>MISKRIARLSDKVRNTQPTIDLDRARLITEFYSRPSMDNYILRRAKAFDYYLENREIFIDEDSQIAGHQGGCWEAVVMHPDVTKWLYDDFDTLDKRPSDNLAFRSAAAKEELRQIVETWKGQTFGDFAATLVDEDMKPMLDVGIFTHGISNQSTMNHSPDYDNLIKRGYRYYIDECKEKLAEHQVNDVYDMEQQIAWKAMIIAMEAVIKFAHRYADLANKQAAECIDPKRKEELLIMAENCRTVPENPPKTFLQATQLVWFNHLAISLEAAGGDHNLGRYDQYMLPFFEKETAEGKPEEYFADIIHEFKLKVAEMWNIRCYNESVADPGNPLWMHIMLAGQLENGKDACNELTNVFLRCMRDLQTDEPCITFRFHPNINEETFRLAIEVARDSGGHPAFYNDTAAITYLLSLGFTLKEARNWGICGCIEPQVLGKTDFQSNPGYFNPLKVFDVMLHNGYDPVIGKKIGIESGEVSSFTSIDDVMRAYEKQLDFFMEKFVTLANRTLAGHAFTLPTIMGSCFSVGCVEKGKLLQQKGSDHHYSAVGVAGIANMIDSFAAMEECVFNKNYLTMEELVRLLDTNFEGKENMRQLLLNKAPKFGNDIEQVDKYSYWLIDALDTSMKRFHDAQGGPYTVLVATQAYNVEMGKNVGATPDGRMAGTPLADNASPMVGMDVNGPTA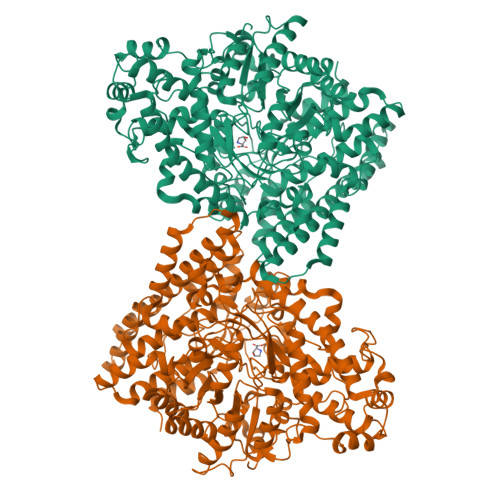VVNSLACCDELVPQSGLLLNQRFDPAVVAGEKGIDIIESVFRAHFAQNGFHIQINVLDDETLRAAQKNPDDHRNILVRVAGYSAYFVDLSEEIQNNIIERTIQRGL[2x]> MSGAAAASAAGYDRHITIFSPEGRLYQVEYAFKATNQTNINSLAVRGKDCTVVISQKKVPDKLLDPTTVSYIFCISRTIGMVVNGPIPDARNAALRAKAEAAEFRYKYGYD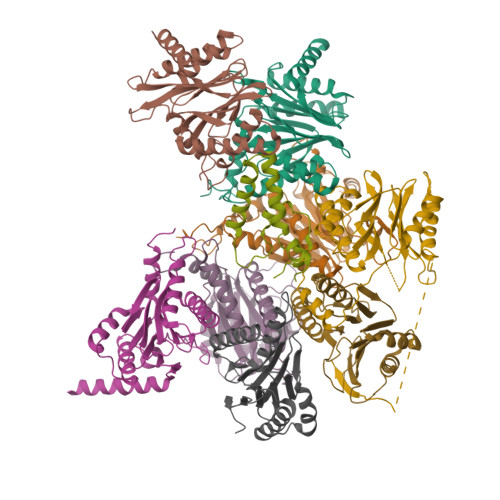MPCDVLAKRMANLSQIYTQRAYMRPLGVILTFVSVDEELGPSIYKTDPAGYYVGYKATATGPKQQEITTNLENHFKKSKIDHINEESWEKVVEFAITHMIDALGTEFSKNDLEVGVATKDKFFTLSAENIEERLVAIAEQD;> MTDRYSFSLTTFSPSGKLGQIDYALTAVKQGVTSLGIKATNGVVIATEKKSSSPLAMSETLSKVSLLTPDIGAVYSGMGPDYRVLVDKSRKVAHTSYKRIYGEYPPTKLLVSEVAKIMQEATQSGGVRPFGVSLLIAGHDEFNGFSLYQVDPSGSYFPWKATAIGKGSVAAKTFLEKRWNDELELEDAIHIALLTLKESVEGEFNGDTIELAIIGDENPDLLGYTGIPTDKGPRFRKLTSQEINDRLEAL;> MGSRRYDSRTTIFSPEGRLYQVEYALESISHAGTAIGIMASDGIVLAAERKVTSTLLEQDTSTEKLYKLNDKIAVAVAGLTADAEILINTARIHAQNYLKTYNEDIPVEILVRRLSDIKQGYTQHGGLRPFGVSFIYAGYDDRYGYQLYTSNPSGNYTGWKAISVGANTSAAQTLLQMDYKDDMKVDDAIELALKTLSKTTDSSALTYDRLEFATIRKGANDGEVYQKIFKPQEIKDILVKTGITKKDEDEEADEDMK;> MSGYDRALSIFSPDGHIFQVEYALEAVKRGTCAVGVKGKNCVVLGCERRSTLKLQDTRITPSKVSKIDSHVVLSFSGLNADSRILIEKARVEAQSHRLTLEDPVTVEYLTRYVAGVQQRYTQSGGVRPFGVSTLIAGFDPRDDEPKLYQTEPSGIYSSWSAQTIGRNSKTVREFLEKNYDRKEPPATVEECVKLTVRSLLEVVQTGAKNIEITVVKPDSDIVALSSEEINQYVTQIEQEKQEQQEQDKKKKSNH;> MTSIGTGYDLSNSVFSPDGRNFQVEYAVKAVENGTTSIGIKCNDGVVFAVEKLITSKLLVPQKNVKIQVVDRHIGCVYSGLIPDGRHLVNRGREEAASFKKLYKTPIPIPAFADRLGQYVQAHTLYNSVRPFGVSTIFGGVDKNGAHLYMLEPSGSYWGYKGAATGKGRQSAKAELEKLVDHHPEGLSAREAVKQAAKIIYLAHEDNKEKDFELEISWCSLSETNGLHKFVKGDLLQEAIDFAQKEINGDDDEDEDDSDNVMSSDDENAPVATNANATTDQEGDIHLE;> MAGLSFDNYQRNNFLAENSHTQPKATSTGTTIVGVKFNNGVVIAADTRSTQGPIVADKNCAKLHRISPKIWCAGAGTAADTEAVTQLIGSNIELHSLYTSREPRVVSALQMLKQHLFKYQGHIGAYLIVAGVDPTGSHLFSIHAHGSTDVGYYLSLGSGSLAAMAVLESHWKQDLTKEEAIKLASDAIQAGIWNDLGSGSNVDVCVMEIGKDAEYLRNYLTPNVREEKQKSYKFPRGTTAVLKESIVNICDIQEEQVDITA;> MSDPSSINGGIVVAMTGKDCVAIACDLRLGSQSLGVSNKFEKIFHYGHVFLGITGLATDVTTLNEMFRYKTNLYKLKEERAIEPETFTQLVSSSLYERRFGPYFVGPVVAGINSKSGKPFIAGFDLIGCIDEAKDFIVSGTASDQLFGMCESLYEPNLEPEDLFETISQALLNAADRDALSGWGAVVYIIKKDEVVKRYLKMRQD;> MDIILGIRVQDSVILASSKAVTRGISVLKDSDDKTRQLSPHTLMSFAGEAGDTVQFAEYIQANIQLYSIREDYELSPQAVSSFVRQELAKSIRSRRPYQVNVLIGGYDKKKNKPELYQIDYLGTKVELPYGAHGYSGFYTFSLLDHHYRPDMTTEEGLDLLKLCVQELEKRMPMDFKGVIVKIVDKDGIRQVDDFQAQ;> MNIVPQDTFKSQVSTDQDKSVLSSAVPSLPDTLRQQEGGAVPLSTQLNDRHPLESTLKNWETTQRQRQMEQYRQIFGIAEPMKRTMEMEIVNRTDFNPLSTNGSIHRDILLNKECSIDWEDVYPGTGLQASTMVGDDVHSKIEKQLGIGRRIPGLINPWKRRWKKNFIAVSAANRFKKISSSGALDYDIPTTASENLYFQ>[2x]MYYLGKELQKRSEELSRGFYELVYPPVDM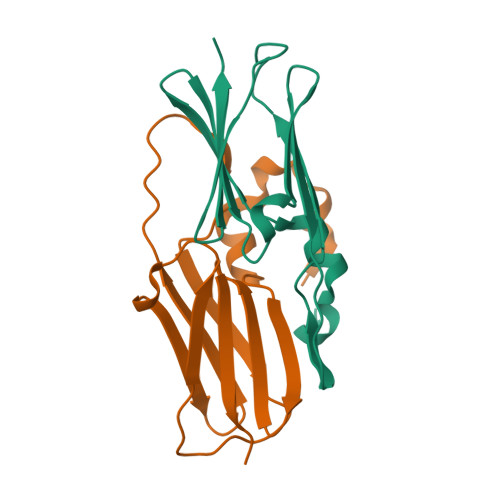YEEGGYLVVVADLAGFNKEKIKARVSGQNELIIEAEREITEPGVKYLTQRPKYVRKVIRLPYNVAKDAEISGKYENGVLTIRIPIA>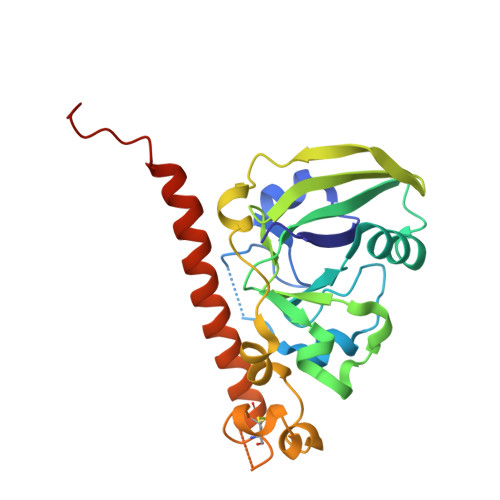 NDDKLYRADSRPPDEIKQSGGLMPRGQSEYFDRGTQMNINLYDHARGTQTGFVRHDDGYVSTSISLRSAHLVGQTILSGHSTYYIYVIATAPNMFNVNDVLGAYSPHPDEQEVSALGGIPYSQIYGWYRVHFGVLDEQLHRNRGYRDRYYSNLDIAPAADGYGLAGFPPEHRAWREEPWIHHAPPGCGNAPRSSMSNTCDEKTQSLGVKFLDEYQSKVKRQIFSGYQSDIDTHNRIKDEL>MKIVLVLYDAGKHAADEEKLYGCTENKLGIANWLKDQGHELITTSDKEGGNSVLDQHIPDADIIITTPFHPAYITKERIDKAKKLKLVVVAGVGSDHIDLDYINQTGKKISVLEVTGSNVVSVAEHVLMTMLVLVRNFVPAHEQIINHDWEVAAIAKDAYDIEGKTIATIGAGRIGYRVLERLVPFNPKELLYYDYQALPKDAEEKVGARRVENIEELVAQADIVTINAPLHAGTKGLINKELLSKFKKGAWLVNTARGAICVAEDVAAALESGQLRGYGGDVWFPQPAPKDHPWRDMRNKYGAGNAMTPHYSGTTLDAQTRYAEGTKNILESFFTGKFDYRPQDIILLNGEYITKAYGKHD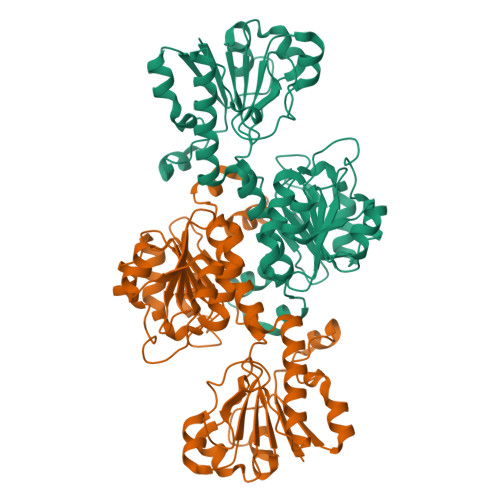KK[4x]> HISLNPDLANEDEVNSCDYWRHCAVDGFLCSCCGGTTTTCPPGSTPSPISWIGTCHNPHDGKDYLISYHDCCGKTACGRCQCNTQTRERPGYEFFLHN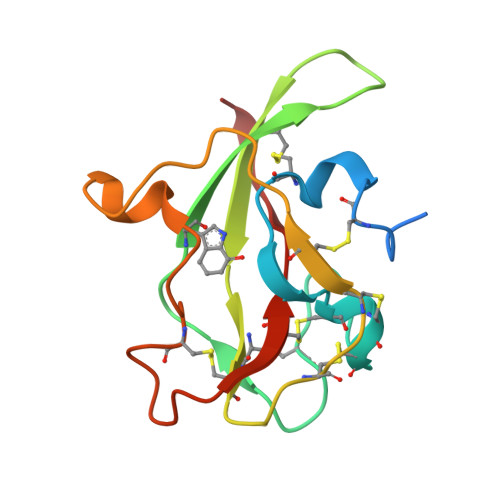DVNWCMANENSTFHCTTSVLVGLA>STFAYIANSESDNISVIDVTSNKVTATIPVGSNPMGAVISPDGTKVYVANAHSNDVSIIDTATNNVIATVPAGSSPQGVAVSPDGKQVYVTNMASSTLSVIDTTSNTVAGTVKTGKSPLGLALSPDGKKLYVTNNGDKTVSVINTVTKAVINTVSVGRSPKGIAVTPDGTKVYVANFDSMSISVIDTVTNSVIDTVKVEAAPSGIAVNPEGTKAYVTNVDKYFNTVSMIDTGTNKITARIPVGPDPAGIAVTPDGKKVYVALSFCNTVSVIDTATNTI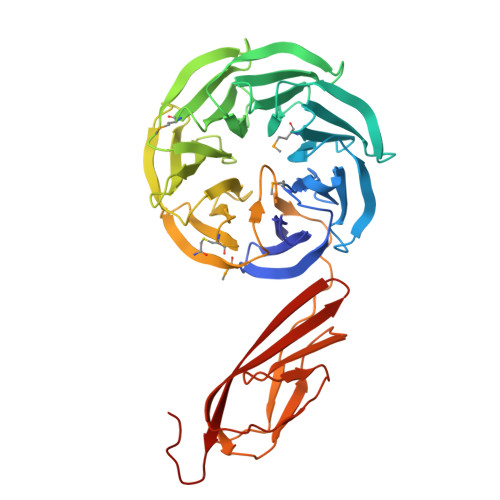TATMAVGKNPYASGQFIGSIPVQPVYPSADFKSNITSGYIFLSEPVQFTDLSKDATEWKWDFGDGSSSKKQNPTHTYSETGIYTVRLTVSNSNGTDSQISTVNVVLKGSPTPS[4x]2-(2-(4-PHENYLPIPERIDIN-1-YL)ETHYL)-1H-INDOLE | C21 H24 N2 | 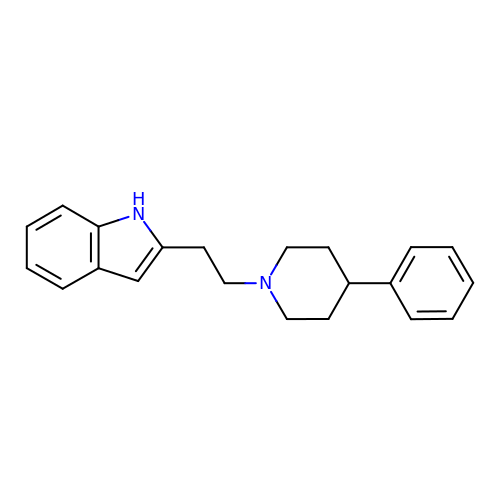PXWYOBGHDFLUNG-UHFFFAOYSA-N> MSNYPLHQACMENEFFKVQELLHSKPSLLLQKDQDGRIPLHWSVSFQAHEITSFLLSKMENVNLDDYPDDSGWTPFHIACSVGNLEVVKSLYDRPLKPDLNKITNQGVTCLHLAVGKKWFEVSQFLIENGAS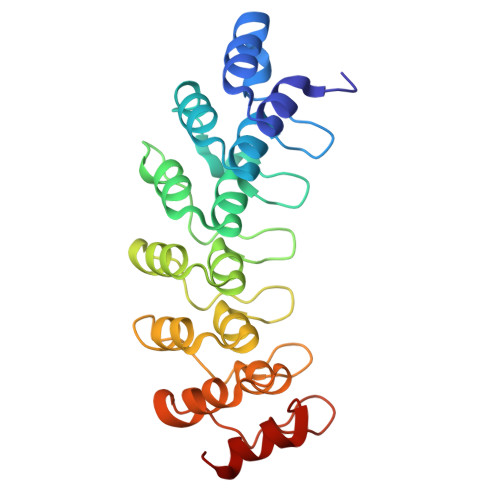VRIKDKFNQIPLHRAASVGSLKLIELLCGLGKSAVNWQDKQGWTPLFHALAEGHGDAAVLLVEKYGAEYDLVDNKGAKAEDVALNEQVKKFFLNNV> GGGCCCGUAGCUCAGUCUGGCAGAGCGCCUGGCUUUUAACCAGGUGGUCGAGGGUUCAAAUCCCUUCGGGCCCGCCA

The KEOPS complex, which is conserved across archaea and eukaryotes, is composed of four core subunits; Pcc1, Kae1, Bud32 and Cgi121. Kae1 catalyzes the universal and essential tRNA modification N6-threonylcarbamoyl adenosine, but the precise roles of all other KEOPS subunits remain an enigma. Here we show using structure-guided studies that Cgi121 recruits tRNA to KEOPS by binding to its 3’ CCA tail. A composite model of KEOPS bound to tRNA reveals that all KEOPS subunits form an extended tRNA-binding surface that we have validated in vitro and in vivo to mediate the interaction with the tRNA substrate and its modification.

Apo-mjtRNALysUUU displays a canonical L-shaped fold that is essentially unchanged in binding to mjCgi121 (RMSD = 1 Å over 64 nucleotides) with two exceptions. Firstly, the conformation of the single-stranded 3′ terminus (G73-A76), which is known to be highly flexible, adopts a specific conformation in response to direct binding to mjCgi121. Secondly, a portion of the anticodon loop is disordered in the tRNA–Cgi121 co-structure. This region is normally stabilized by t6A17 and its ordered nature in the apo–tRNA structure appears to be due to crystal packing interactions.> MSHPIQFVNANNSDKSHQLGGQYSIPQDLRENLQKEAARIGENEKDVLQEKMETRTVQNREDSYHKRRFDMKFEPDSDTQTVTSSENTQDAVVPRKRKSRWDVKGYEPPDESSTAVKENSDSALVNVEGIHDLMFFKPSDHKYFADVISKKPIDELNKDEKKERTLSMLLLKIKNGNTASRRTSMRILTDKAVTFGPEMIFNRLLPILLDRSLEDQERHLMIKTIDRVLYQLGDLTKPYVHKILVVAAPLLIDEDPMVRSTGQEIITNLSTVAGLKTILTVMRPDIENEDEYVRNVTSRAAAVVAKALGVNQLLPFINAACHSRKSWKARHTGIKIVQQIGILLGIGVLNHLTGLMSCIKDCLMDDHVPVRIVTA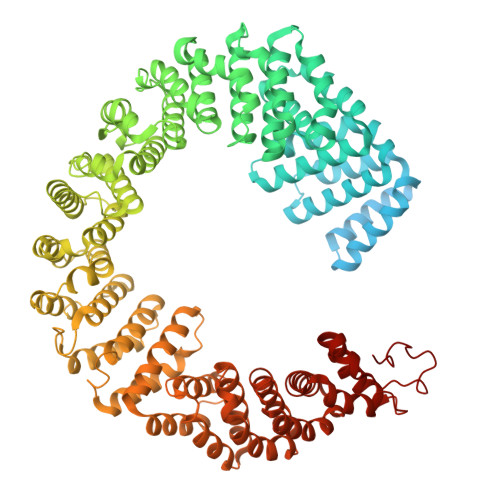HTLSTLAENSYPYGIEVFNVVLEPLWKGIRSHRGKVLSSFLKAVGSMIPLMDPEYAGYYTTEAMRIIRREFDSPDDEMKKTILLVLQKCSAVESITPKFLREEIAPEFFQKFWVRRVALDRPLNKVVTYTTVTLAKKLGCSYTIDKLLTPLRDEAEPFRTMAVHAVTRTVNLLGTADLDERLETRLIDALLIAFQEQTNSDSIIFKGFGAVTVSLDIRMKPFLAPIVSTILNHLKHKTPLVRQHAADLCAILIPVIKNCHEFEMLNKLNIILYESLGEVYPEVLGSIINAMYCITSVMDLDKLQPPINQILPTLTPILRNKHRKVEVNTIKFVGLIGKLAPTYAPPKEWMRICFELLELLKSTNKEIRRSANATFGFIAEAIGPHDVLVALLNNLKVQERQLRVCTAVAIGIVAKVCGPYNVLPVIMNEYTTPETNVQNGVLKAMSFMFEYIGNMSKDYIYFITPLLEDALTDRDLVHRQTASNVITHLALNCSGTGHEDAFIHLMNLLIPNIFETSPHAIMRILEGLEALSQALGPGLFMNYIWAGLFHPAKNVRKAFWRVYNNMYVMYQDAMVPFYPVTPDNNEEYIEELDLVL> PKHLTRYLPFVPTSLVHETTSFLHDATKLRALLALIFSPCKPEASVADELASPAARLEFQQEKERYHAIRDQHTDCYRRHESAAAASM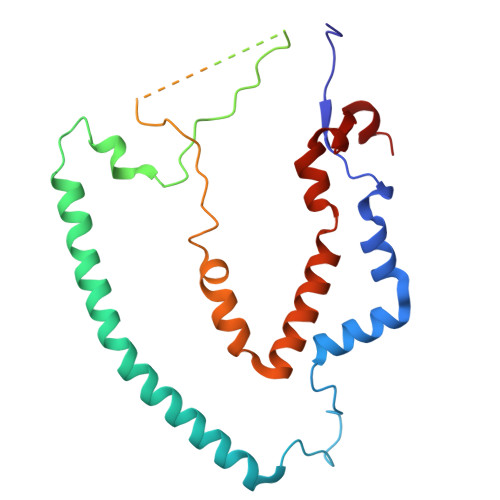WRAIEALPSDLYEEAVQSVTFAPPYENEPPPPDPSELRPGKNASTETQAASAGQQPSAASRGSSVRTLAGPGAAGEAVSQPEHGFYHERFAFPRALMFHEMYGEQIFQSLSQLERRKLQVFMNLMHVRYPHAELKRDKPALFWLPERQVLSR> MQPWGRLLRLGAEEGEPHVLLRKREWTIGRRRGCDLSFPSNKLVSGDHCRIVVDEKSGQVTLEDTSTSGTVINKLKVVKKQTCPLQTGDVIYLVYRKNEPEHNVAYLYESLSEKQ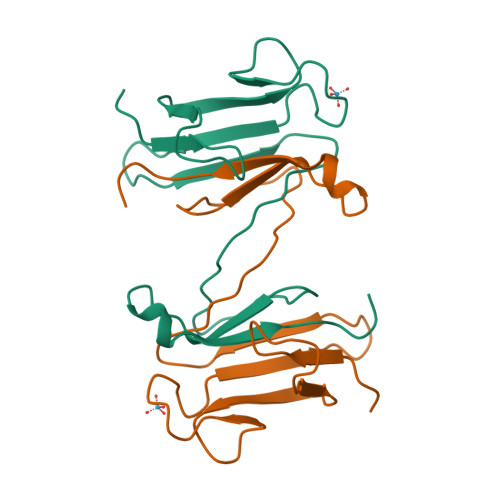G6-(but-3-en-1-yl)-4-[3-(morpholine-4-carbonyl)phenyl]-1,6-dihydro-7H-pyrrolo[2,3-c]pyridin-7-one 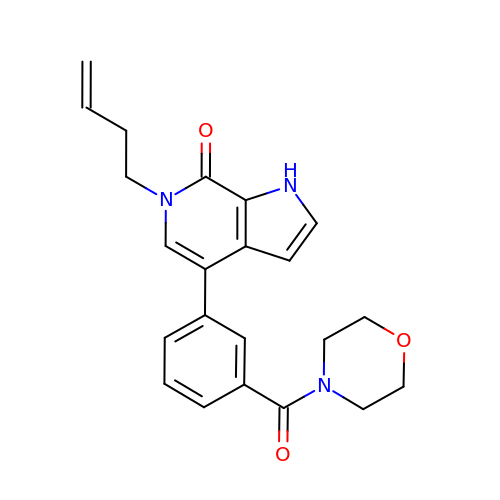| C22 H23 N3 O3 | SMABWKWHQKFGDR-UHFFFAOYSA-N> GIEETIDTVITNALQLSQPKPQKQPTAQSTPLTSGVNSQEVPALTAVETGASGQAVPSDVIETRHVVNYKTRSESTLESFFGRSACVTILEVENFNATTDADRKKQFTTWAITYTDTVQLRRKLEFFTYSRFDLEMTFVITERYYASNTGHARNQVYQLMYIPPGAPRPTAWDDYTWQSSSNPSVFYTYGSAPPRMSIPYVGIANAYSHFYDGFARVPLKDETVDSGDTYYGLVTINDFGTLAVRVVNEYNPARITSKIRVYMKPKHVRCWCPRPPRAVPYRGEGVDFKQDSITPLTAVENINTF;> SPNVEACGYSDRVRQITLGNSTITTQEAANAVVAYGEWPSYLDDKEANPIDAPTEPDVSSNRFYTLDSVQWKSTSRGWWWKLPDALKDMGMFGQNMYYHYLGRSGYTVHVQCNASKFHQGALGVFAIPEYVMACNTEAKTSYVSYVNANPGEKGGVFDNAYNPSAEASEGRKFAALDYLLGCGVLAGNAFVYPHQIINLRTNNSATLVLPYVNSLAIDCMAKHNNWGLVILPLCKL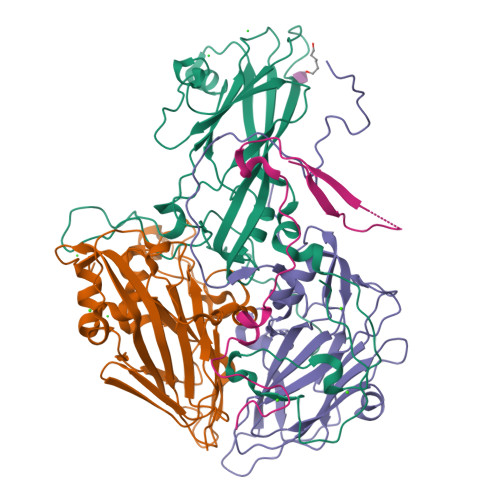DYAPNSSTEIPITVTIAPMFTEFNGLRNITVPATQ;> GLPTMLTPGSSQFLTSDDFQSPCALPNFDVTPPIHIPGEVFNMMELAEIDSMIPMNSVTGKANTMEMYPIPLDDKGSATPIFSISLSPASDKRLQYTMLGEILNYYTHWTGSLRFTFLFCGSMMATGKILLSYSPPGAKPPTTRKDAMLGTHIIWDLGLQSSCTMLAPWISNTVYRRCIKDDFTEGGYITCFYQTRIVVPSGTPTSMFMLAFVSACPDFSVRLLRDTNHISQRTLFARAQ;> MGAQVSSQKVGAHENTNVATGGSTVNYTTINYYKDSASNAASKLDFSQDPSKFTEPVKDIMIKTAPALN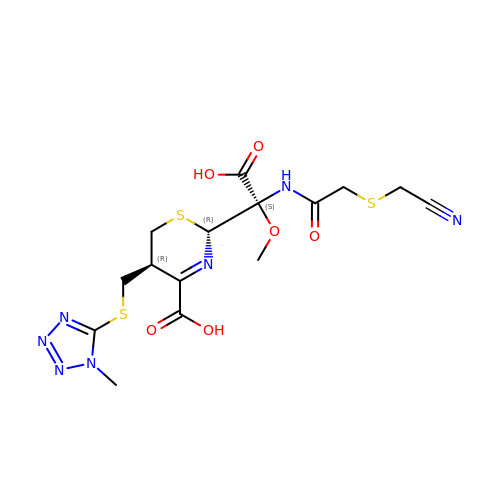(2R,5R)-2-[(1S)-1-[2-(cyanomethylsulfanyl)ethanoylamino]-1-methoxy-2-oxidanyl-2-oxidanylidene-ethyl]-5-[(1-methyl-1,2,3,4-tetrazol-5-yl)sulfanylmethyl]-5,6-dihydro-2H-1,3-thiazine-4-carboxylic acid | C15 H19 N7 O6 S3 | VZQGYYZNCGIOGL-AOAMOSOWSA-N>[2x]SNAMNFKESRAIYLQIADRICDDILLGQYEEEGRIPSVREYASIVEVNANTVMRSYEYLQSQEVIYNKRGIGFFVASGAKMLIHSLRKEQFLKEEVGSFFRQLYTLGISI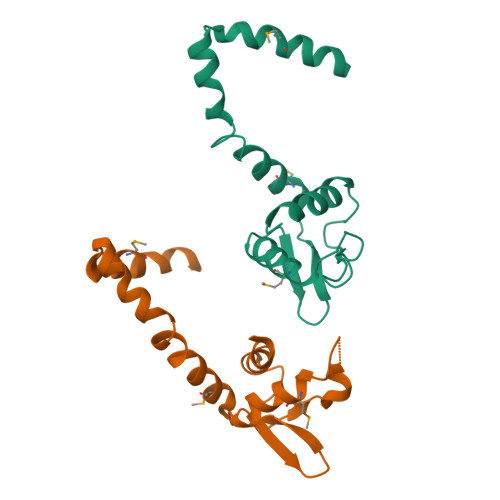KEIEKMYYEFIQRQNQ>GAMEAIYAYEAQGDDEISIDPGDIITVIRGDDGSGWTYGECDGLKGL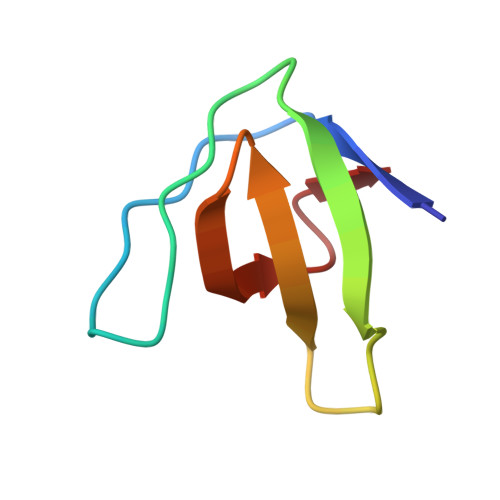FPTSYCK[4x]>MPATHHSSATSAERPTVVGRIPVLDVRPVVQRGRRPAKAVTGESFEVSATVFREGHDAVGANVVLRDPRGRPGPWTPMRELAPGTDRWGATVTAGETGTWSYTVEAWGDPVTTWRHHARIKIPAGLDTDLVLEEGARLYERAAADVPGREDRRELLAAVDALRDESRPAASRLAAALTPQVDAVLARHPLRDLVTSSDPLPLLVERERALYGAWYEFFPRSEGTPHTPHGTFRTAARRLPAIAAMGFDVVYLPPIHPIGTTHRKGRNNTLSATGDDVGSPWAIGSPEGGHDS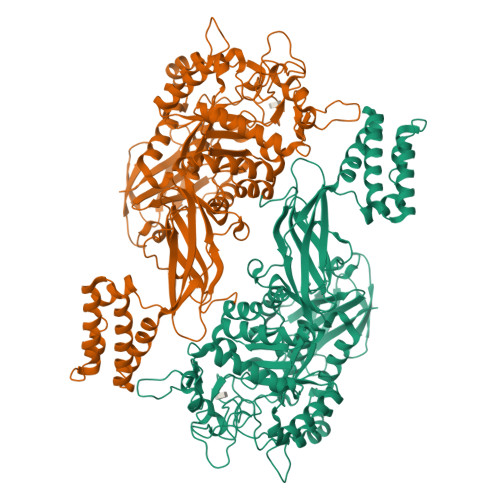IHPALGTLDDFDHFVTEAGKLGLEIALDFALQCSPDHPWVHKHPEWFHHRPDGTIAHAENPPKKYQDIYPIAFDADPDGLATETVRILRHWMDHGVRIFRVDNPHTKPVAFWERVIADINGTDPDVIFLAEAFTRPAMMATLAQIGFQQSYTYFTWRNTKQELTEYLTELSGEAASYMRPNFFANTPDILHAYLQHGGRPAFEVRAVLAATLSPTWGIYSGYELCENTPLREGSEEYLDSEKYQLKPRDWTRAAREGTTIAPLVTRLNTIRRENPALRQLRDLHFHPTDKEEVIAYSKRQGSNTVLVVVNLDPRHTQEATVSLDMPQLGLDWHESVPVRDELTGETYHWGRANYVRLEPGRTPAHVCTVLR[4x]> MDPEDELKRVEKLVKEAEELLRQAKEKGSEEDLEKALRTAEEAAREAKKVLEQAEKEGDPEVALRAVELVVRVAELLLRIAKESGSEEALERALRVAEEAARLAKRVLELAEKQGDPEVALRAVELVVRVAELLLRIAKESGSEEALERALRVAEEAARLAKRVLELAEKQGDPEVARRAVELVKRVAELLERIARESGSEEAKERAERVREEARELQERVKELREREGGWLEHHHH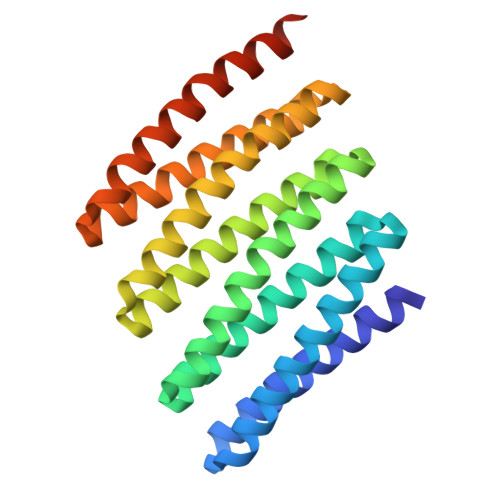HH>GAMVYTVSYDVDGTVIKTKVEAGTRITAPKPP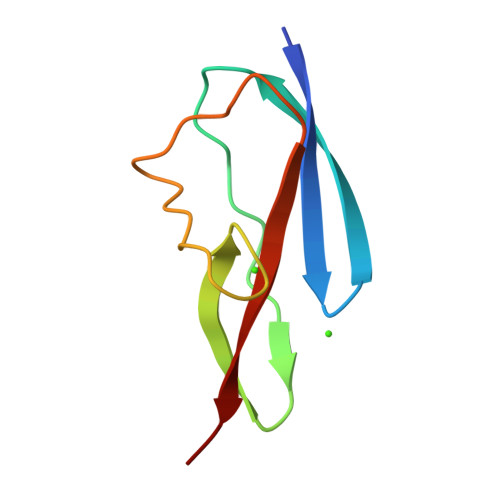TKQGYVFKGWYTEKNGGHEWNFNTDYMSGNDFTLYAVFKAET[4x]> GIGKFLH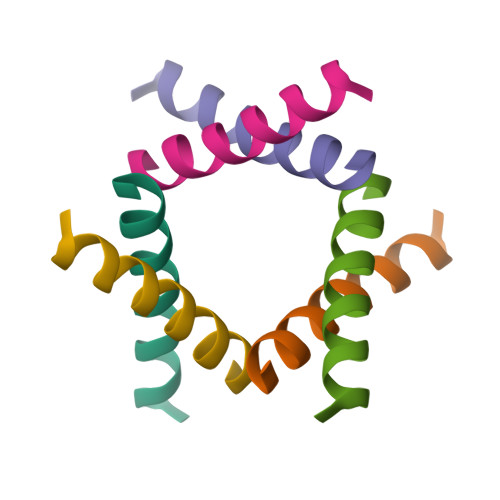SAKKFGKAFVGEIMNS N-[(2S)-3-(3,5-difluorophenyl)-1-[[(3S,9S,13S,15R,19S,22S)-15,19-dimethyl-2,8,12,18,21-pentaoxo-11-oxa-1,7,17,20-tetrazatetracyclo[20.4.0.03,7.013,17]hexacosan-9-yl]amino]-1-oxopropan-2-yl]heptanamide 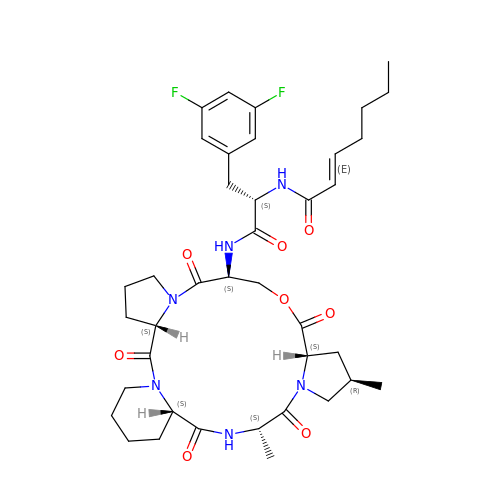| C39 H52 F2 N6 O8 | BAEUBYUDIYWBPI-CSGPBTBZSA-N> MNPFHELEPGPEVPEVVYALIEIPKGSRNKYELDKKTGLLKLDRVLYSPFFYPVDYGIIPQTWYDDGDPFDIMVIMREPVYPLTIIEARPIGIMKMEDSGDKDWKVLAVPVEDPYFND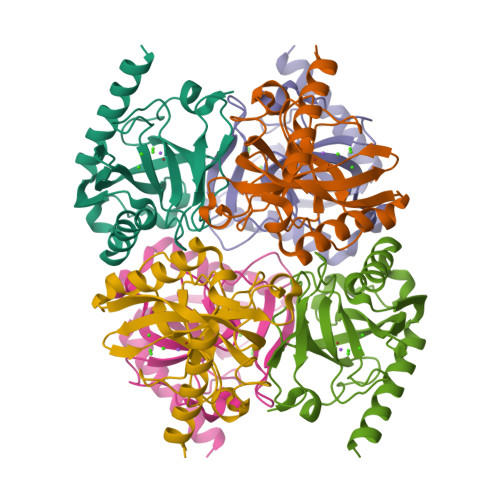WKDISDVPKAFLDEIAHFFQRYKELQGKTTKIEGWGNAEEAKREILRAIEMYKEKFGKEE> MSLSFCGNNISSYNIYHGVLQNPCFVDALNLVPHVFLLFITFPILFIGWGSQSSKVQIHHNTWLHFPGHNLRWILTFALLFVHVCEIAEGIVSDSQRASRHLHLFMPAVMGFVATTTSIVYYHNIETSNFPKLLLALFLYWVMAFITKTIKLVKYWQLGWGMSDLRFCITGVMVILNGLLMAVEINVIRVRRYVFFMNPQKVKPPEDLQDLGVRFLQPFVNLLSKATYWWMNTLIISAHRKPIDLKAIGKLPIAMRAVTNYVCLKEAYEEQKKKAADHPNRTPSIWLAMYRAFGRPILLSSTFRYLADLLGFAGPLCISGIVQRVNEPKNNTTRFSETLSSKEFLENAHVLAVLLFLALILQRTFLQASYYVTIETGINLRGALLAMIYNKILRLSTSNLSMGEMTLGQINNLVAIETNQLMWFLFLCPNLWAMPVQIIMGVILLYNLLGSSALVGAAVIVLLAPIQYFIATKLAEAQKSTLDYSTERLKKTNEILKGIKLLKLYAWEHIFCKSVEETRMKELSSLKTFALYTSLSIFMNAAIPIAAVLATFVTHAYASGNNLKPAEAFASLSLFHILVTPLFLLSTVVRFAVKAIISVQKLNEFLLSDEIGEDSWRTGEGTLPFESCKKHTGVQSKPINRKQPGRYHLDNYEQARRLRPAETEDVAIKVTNGYFSWGSGLATLSNIDIRIPTGQLTMIVGQVGCGKSSLLLAILGEMQTLEGKVYWNNVNESEPSFEATRSRSRYSVAYAAQKPWLLNATVEENITFGSSFNRQRYKAVTDACSLQPDIDLLPFGDQTEIGERGINLSGGQRQRICVARALYQNTNIVFLDDPFSALDIHLSDHLMQEGILKFLQDDKRTVVLVTHKLQYLTHADWIIAMKDGSVLREGTLKDIQTKDVELYEHWKTLMNRQDQELEKDMEADQTTLERKTLRRAMYSREAKAQMEDEDE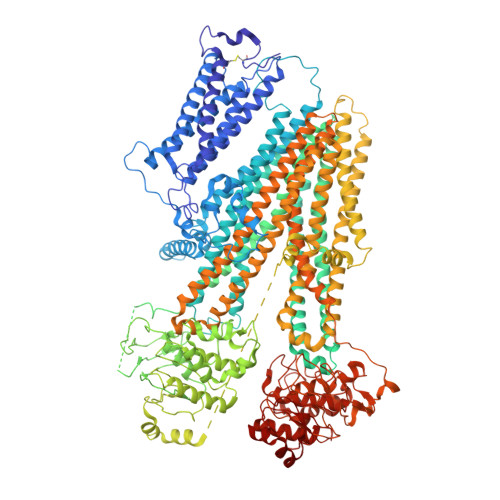EEEEEEDEDDNMSTVMRLRTKMPWKTCWWYLTSGGFFLLFLMIFSKLLKHSVIVAIDYWLATWTSEYSINDPGKADQTFYVAGFSILCGAGIFLCLVTSLTVEWMGLTAAKNLHHNLLNKIILGPIRFFDTTPLGLILNRFSADTNIIDQHIPPTLESLTRSTLLCLSAIGMISYATPVFLIALAPLGVAFYFIQKYFRVASKDLQELDDSTQLPLLCHFSETAEGLTTIRAFRHETRFKQRMLELTDTNNIAYLFLSAANRWLEVRTDYLGACIVLTASIASISGSSNSGLVGLGLLYALTITNYLNWVVRNLADLEVQMGAVKKVNSFLTMESENYEGTMDPSQVPEHWPQEGEIKIHDLCVRYENNLKPVLKHVKAYIKPGQKVGICGRTGSGKSSLSLAFFRMVDIFDGKIVIDGIDISKLPLHTLRSRLSIILQDPILFSGSIRFNLDPECKCTDDRLWEALEIAQLKNMVKSLPGGLDATVTEGGENFSVGQRQLFCLARAFVRKSSILIMDEATASIDMATENILQKVVMTAFADRTVVTIAHRVHTILTADLVIVMKRGNILEYDTPESLLAQEDGVFASFVRADM>GSHMASSCAVQVKLELGHRAQVRKKPTVEGFTHDWMVFVRGPEHSNIQHFVEKVVFHLHESFPRPKRVCKDPPYKVEESGYA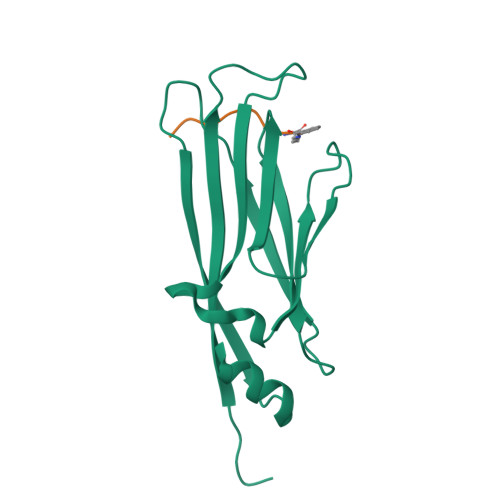GFILPIEVYFKNKEEPRKVRFDYDLFLHLEGHPPVNHLRCEKLTFNNPTEDFRRKLLKA[2x];>[2x]TKQTARKS> GMPTFNPELHAQTLNSERAYFVQPDADPAFTPHIGALVEMLTYARLTTLQAVEGLPEDQLWATAPGFANSIGTLLAHIAAVERVYHVLSFQGRDVTPEDDGAAYWGLT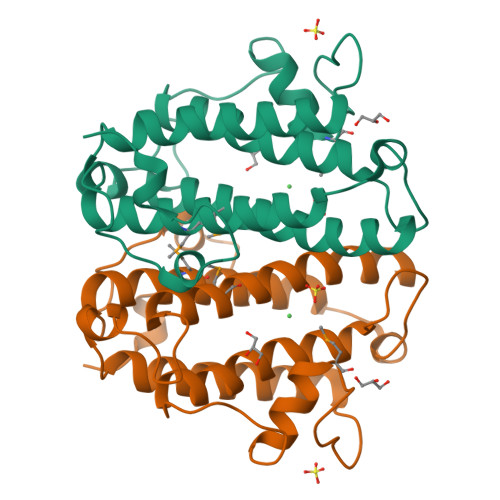MGKEGTAPARLPTLDELRAELADARAETLRVFAAKDDAWLAEPLGPGWANQHWAWFHVMEDEVNHRGQLRLLRQVLAPEEGG>[2x]GSHGGSMLTILKLGGSILSDKNVPYSIKWDNLERIAMEIKNALDYYKNQNKEIKLILVHGGGAFGHPVAKKYLKIEDGKKIFINMEKGFWEIQRAMRRFNNIIIDTLQSYDIPAVSIQPSSFVVFGDKLIFDTSAIKEMLKRNLVPVIHGDIVIDDKNGYRIISGDDIVPYLANELKADLILYATDVDGVLIDNKPIKRIDKNNIYKILNYLSGSNSI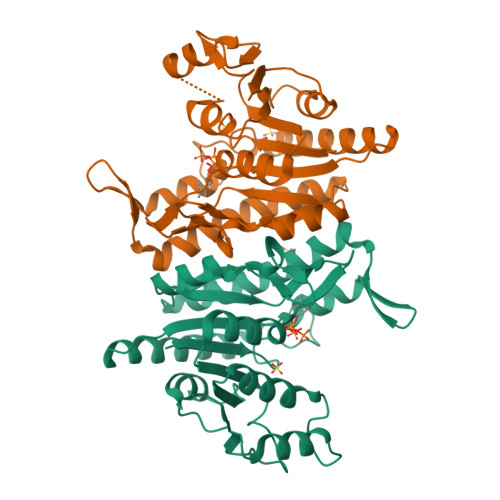DVTGGMKYKIEMIRKNKCRGFVFNGNKANNIYKALLGEVEGTEIDFSE> GPVEDAITAAIGRVADTVGTGPTNSEAIPALTAAETGHTSQVVP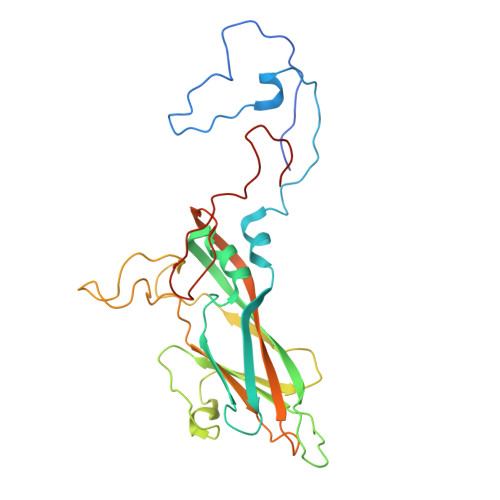GDTMQTRHVKNYHSRSESTIENFLCRSACVYFTEYKNSGAKRYAEWVLTPRQAAQLRRKLEFFTYVRFDLELTFVITSTQQPSTTQNQDAQILTHQIMYVPPGGPVPDKVDSYVWQTSTNPSVFWTEGNAPPRMSIPFLSIGNAYSNFYDGWSEFSRNGVYGINTLNNMGTLYARHVNAGSTGPIKSTIRIYFKPKHVKAWIPRPPRLCQYEKAKNVNFQPSGVTTTRQSITTMTNTGAF>[2x]LPTAQEVQGLMARYIELVDVGD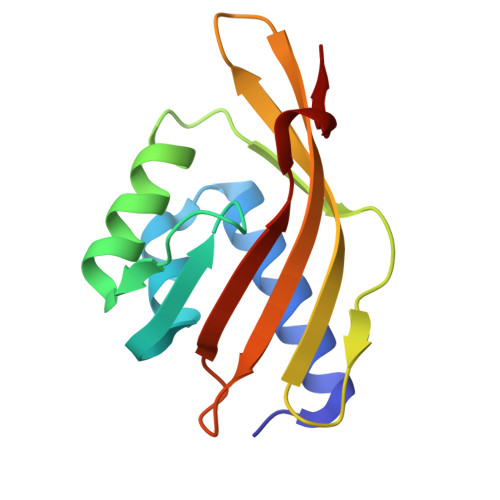IEAIVQMYADDATVEDPFGQPPIHGREQIAAFYRQGLGGGKVRACLTGPVRASHNGCGAMPFRVEMVWNGQPCALDVISVMRFDEHGRIQTMQAYWSEVNLSV> GHMLRLSAPGQLDDDLCLLGDVQVPVFLLRLGEASWALVEGGISRDAELVWADLCRWVADPSQVHYWLITHKHYDHCGLLPYLCPRLPNVQVLASERTCQAWKSESAVRVVERLNRQLLRAEQRLPEACAWDALPVRAVADGEWLELGPRHRLQVIEAHGHSDDHVVFYDVRRRRLFCGDALGEFDEARGVWRPLVFDDMEAYLESLERLQRLPTLLQLIPGHGGLLRGRLAADGAESAYTECLRLCRRLLWRQSMGESLDELSEELHRAWGGQSVDFLPGELHLGSMRRMLEILSRQALPLD

The majority of traits controlled by rhl transcription factor RhlR depend on PqsE, a dispensable thioesterase in Pseudomonas Quinolone Signal (PQS) biosynthesis that interferes with RhlR through an enigmatic mechanism likely involving direct interaction of both proteins. Here we show that PqsE and RhlR form a 2:2 protein complex that, together with RhlR agonist N-butanoyl-L-homoserine lactone (C4-HSL), solubilizes RhlR and thereby renders the otherwise insoluble transcription factor active. PqsE is a thioesterase that triggers transcription of the RhlR regulon through a hitherto cryptic mechanism, which we identify here as involving a significant chaperone-like component that enhances the stability of RhlR via protein complex formation. In common with many other gram-negative bacteria, two QS circuits use N-acyl-L-homoserine lactones (HSLs) as autoinducers, namely N-(3-oxododecanoyl)-L-HSL (3-oxo-C12-HSL) and N-butanoyl-L-HSL (C4-HSL), which are produced by autoinducer synthases LasI and RhlI and activate the LuxR-type transcription factors LasR and RhlR, respectively.

Interestingly, while the presence of two chains of RhlR was expected since similar transcription factors are homodimeric, PqsE itself was found to be dimeric as well. We, therefore, re-analyzed crystal structures of PqsE in the Protein Data Bank39 and found that PqsE forms similar dimers in all of these entries. After introducing a mutation in the dimer interface (E187R), we could obtain and crystallize a monomeric form of PqsE. The mutation led to strongly reduced production of the PqsE/RhlR-controlled phenazine virulence factor pyocyanin and also weakened the interaction with RhlR significantly, suggesting that dimerization of PqsE is a prerequisite for tight interaction with RhlR. Similar experiments with PqsE-E187R were more difficult to perform due to rapid protein precipitation and yielded an inverse titration curve corresponding to a KD of 13.8 ± 3.9 μM. Impaired dimer formation may also explain the pyocyanin-reducing effect of mutations within α-helices at the C-terminus of PqsE that have recently been observed by others. These α-helices belong to the dimerization motif of PqsE and are unique within the metallo-β-lactamase family.4-[(3-chlorophenyl)methyl]-N-[[(3S)-2,3-dihydro-1,4-benzodioxin-3-yl]methyl]-3-oxidanylidene-1,4-benzothiazine-6-carboxamide 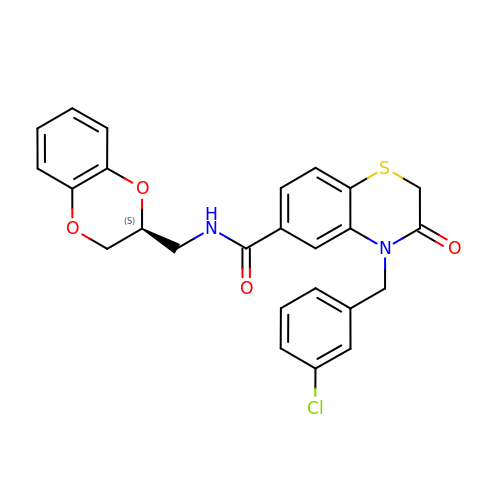| C25 H21 Cl N2 O4 S | JDJXOOKBURTXCO-IBGZPJMESA-N> MLYPVLTQSRLLSDLSGVWDFKLDNGKGFEEKWYEKPLKDADTMPVPASYNDLKEGTDFRDHYGWVFYQRNISVPEYVKSQRIVLRCAAVTHYAMIYLNGKLICEHKGGFLPFEVELNDDLQDGDNLLTIAVNNVIDYTTLPVGGKANMMSGMMGGMGAGASDKPQNNPNFDFFNYCGITRPVKIYTT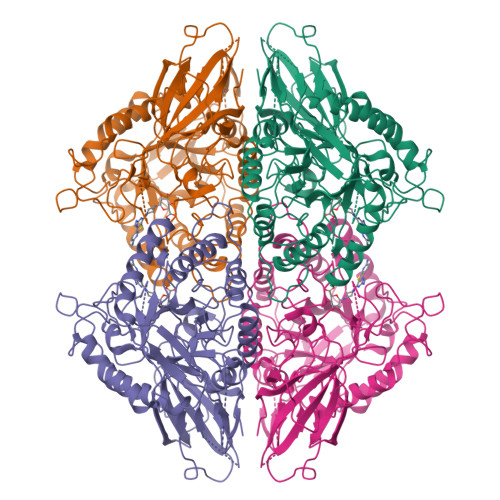PETYINDITVTADIDFTKEEPSAVLNYNVEIKGKDYNNITCKVELFDEEGTKLSETEGSEGTFEISNVRLWQPLNAYLYKIKVTAGQDVYTLPYGVRSVRVDGTKFLINEKPFYFKGYGKHEDTFPNGRGINLPMNTKDISIMKWQHANSFRTSHYPYSEEMMRLCDEEGIVVIDETTAVGVNLQFGGGANFGGERIGTFDKEHGVQTQEHHKDVIRDLISRDKNHACVVMWSIANEPDSAAEGAYDYFKPLYDLARELDPQKRPCTLVSVQGTTADTDCSSQLSDVICLNRYYGWYFGGPDLEVSEIGLRKELSDWGKLGKPVMFTEYGADTVSGLHDTTSVMYTEEYQVEYYEMNNKVFDEFDFVVGEQAWNFADFATSQSLLRVQGNKKGLFTRDRKPKMVAHYFRNRWSTIPEFGYKTK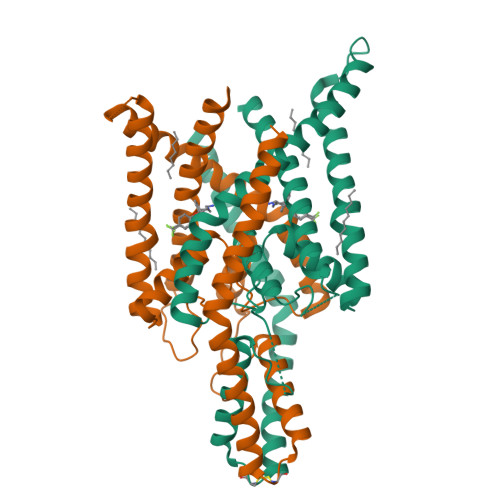>[4x]MGLQTVMKWKTVVAIFVVVVVYLVTGGLVFRALEQPFESSQKNTIALEKAEFLRDHVCVSPQELETLIQHALDADNAGVSPIGNSSNNSSHWDLGSAFFFAGTVITTIGYGNIAPSTEGGKIFCILYAIFGIPLFGFLLAGIGDQLGTIFGKSIARVEKVFRKKQVSQTKIRVISTILFILAGCIVFVTIPAVIFKYIEGWTALESIYFVVVTLTTVGFGDFVAGGNAGINYREWYKPLVWFWILVGLAYFAAVLSMIGDWLRVLSKKTKEEVGEAENLYFQ> MKNNHMQVEAICNGYVIDHIPSGQGVKILKLFSLT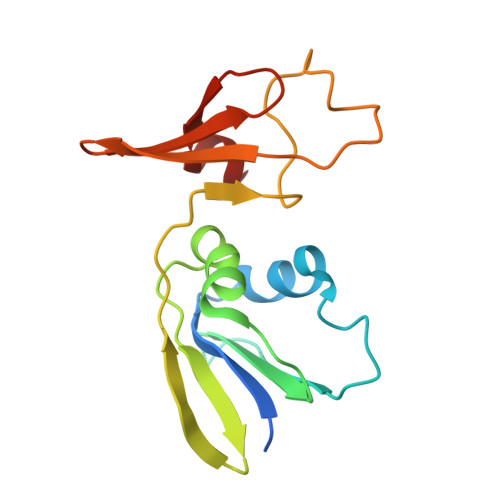DTKQRVTVGFNLPTKDGNAKDLIKVENTEITKSQANQLALLAPNATINIIENFKVTDKHSLTLPNEVENVFPCPNSNCITHGEPVTSSFSIKKTKGNIGLKCKYCEKTFSKDIVTEQV> GPLGSMSEFRIHHDVNELISLLHVFGLEGADVYIDLLQKNRTPYVTTSVSTHSAKVKI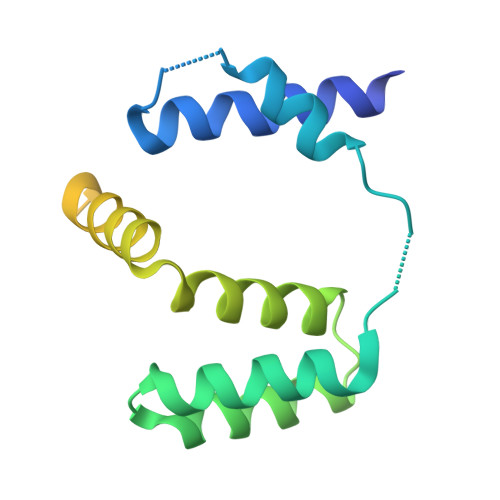AEFSRTPDDFLKKYEELKSKNTRNLDPLVYLLSKLIEDKETLQYLQQNAKDKAELATSSVTSVSLPIAPNTSKISMQELEELRRQLETATVAVSCSHQPVEVLRKFLRDK>HHHMSEATLLSYTKKLLASPPQLSSTDLHDALLVILSLLQKCDTNSDESLSIYTKVSSFLTALRVTKLDHKAEYIAEAAKAVLRHSDLVDLPLPKKDELHPEDGPVILDIVGTGGDGQNTFNVATSAAIVASGIQGLKICKHGGKASTSNSGAGDLIGTLGCDMFKVNSSTVPKLWPDNTFMFLLAPFFHHGMGHVSKIRKFLGIPTVFNVLGPLLHPVSHVNKRILGVYSKELAPEYAKAAALVYPGSETFIVWGHVGLDEVSPIGKTTVWHIDPTSSELKLKTFQLEPSMFGLEEHELSKCASYGPKENARILKEEVLSGKYHLGDNNPIYDYILMNTAVLYCLSQGHQNWKEGIIKAEESIHSGNALRSLEHFIDSVSSL[2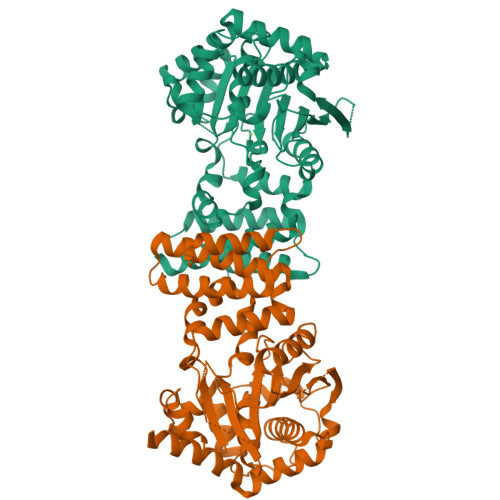x]>[3x]MELPTYRYPLELDTANNRVQVADRFGMRTGTWTGQLQYQHPQLSWRANVTLNLMKVDDWLVLSFSQMTTNSIMADGKFVINFVSGLSSGWQTGDTEPSSTIDPLSTT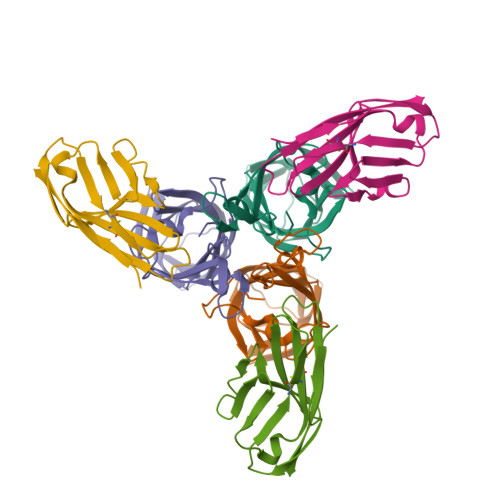FAAVQFLNNGQRIDAFRIMGVSEWTDGELEIKNYGGTYTGHTQVYWAPWTIMYPCNVR;>GSSVTVHSSEPEVRIPENNPVKLSCAYSGFSSPRVEWKFDQGDTTRLVCYNNKITASYEDRVTFLPTGITFKSVTREDTGTYTCMVSEEGGNSYGEVKVKLIVL[3x]> SMSKSKVDNQFYSVEVGDSTFTVLKRYQNLKPIGSGAQGIVCAAYDAVLDRNVAIKKLSRPFQNQTHAKRAYRELVLMKCVNHKNIISLLNVFTPQKTLEEFQDVYLVMELMDANLCQVIQMELDHERMSYLLYQMLCGIKHLHSAGIIHRDLKPSNIVVKSDCTLKILDFGLARTAGTSFMMTPYVVTRYYR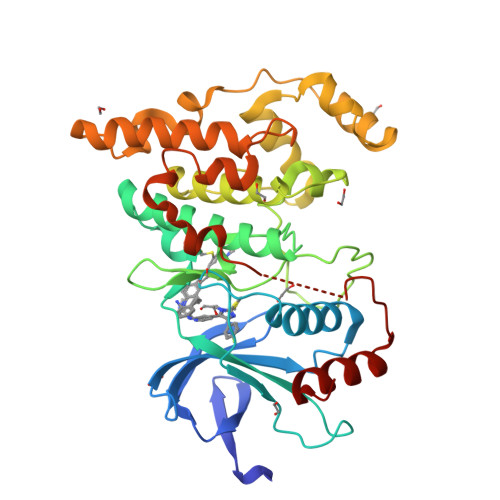APEVILGMGYKENVDIWSVGCIMGEMVRHKILFPGRDYIDQWNKVIEQLGTPCPEFMKKLQPTVRNYVENRPKYAGLTFPKLFPDSLFPADSEHNKLKASQARDLLSKMLVIDPAKRISVDDALQHPYINVWYDPAEVEAPPPQIYDKQLDEREHTIEEWKELIYKEVMNSE>TALAEMPKRKFTIDDFDIGRPLGKGKFGNVYLAREKQNKFIMALKVLFKSQLEKEGVEHQLRREIEIQSHLRHPNILRMYNYFHDRKRIYLMLEFAPRGELYKELQKHGRFDEQRSATFMEELADALHYCHERKVIHRDIKPENLLMGYKGELKIADFGWSVHAPSLRRRTMCGTLDYLPPEMIEGKTHDEKVDLWCAGVLCYEFLVGMPPFDSPSHTETHRRIVNVDLKFPPFLSDGSKDLISKLLRYHPPQRLPLKGVMEHPWVKANSRRVLPPVYQSTQSK[2x];>[2x]IPAWASGNLLTQAIRQQYYKPIDVDRMYGTIDSPKLEEL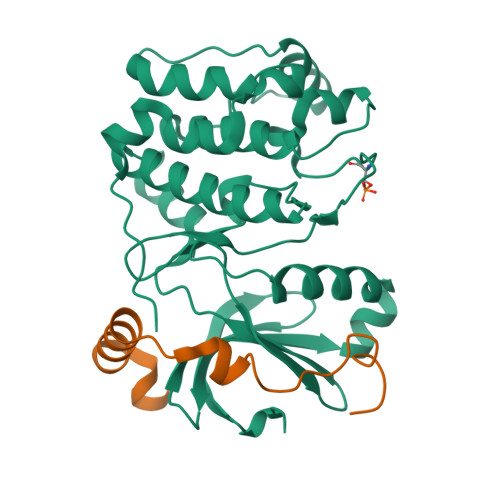FNKS>[14x]GAMAERPLDVIHRS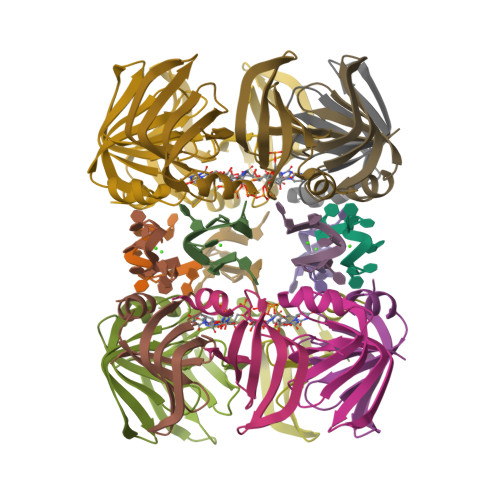LDKDVLVILKKGFEFRGRLIGYDIHLNVVLADAEMIQDGEVVKRYGKIVIRGDNVLAISPTEE> MSIVNILSVNVLNNPAKFSDPYKFEITFECLEPLKSDLEWKLTYVGSATSQSYDQILDTLLVGPIPIGINKFVFEADPPNIDLLPQLSDVLGVTVILLSCAYEDNEFVRVGY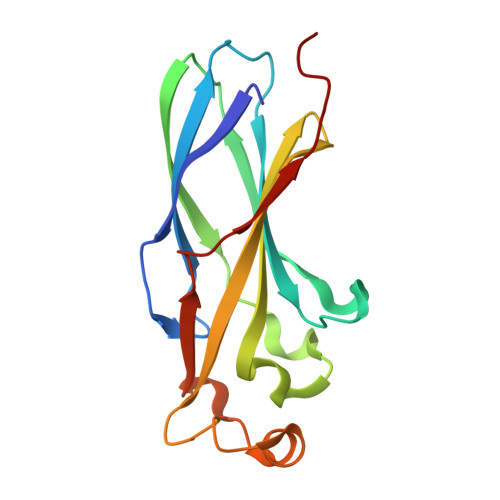YVNNEMEGLNLQEMDDAEIKKVKVDISKVWRSILAEKPRVTRFNIQWDN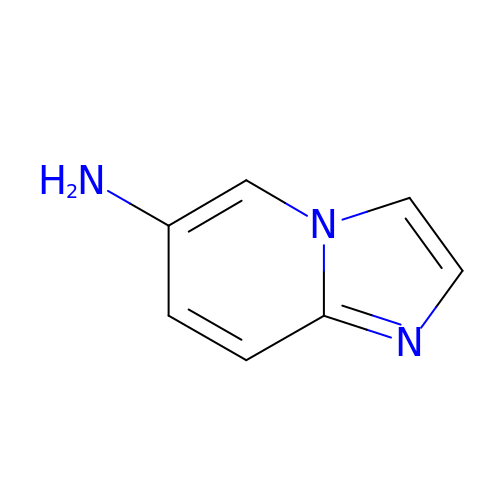imidazo[1,2-a]pyridin-6-amine | C7 H7 N3 | FBEUDMIHYYXAJG-UHFFFAOYSA-N> GSPGILAPLAPGSEDNFARFVCKNNGVLFENQLLQIGLKSEFRQNLGRMFIFYGNKTSTQFLNFTPTLICADDLQTNLNLQTKPVDPTVDGGAQVQQVINIECISDFTEAPVLNIQFRYGGTFQNVSVKLPITLNKFFQPTEMASQDFFQRWKQLSNPQQEVQNIFKAKHPMDTEITKAKIIG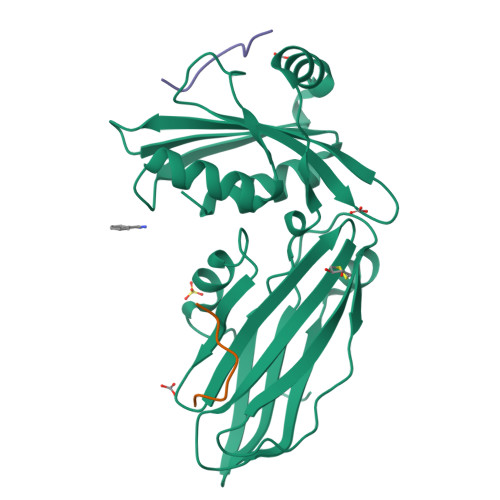FGSALLEEVDPNPANFVGAGIIHTKTTQIGCLLRLEPNLQAQMYRLTLRTSKDTVSQRLCELLSEQF;> NPKGWVTFEEEE;> LDGFKDSFDLQG>[2x]GPSGMILKRAYDVTPQKISTD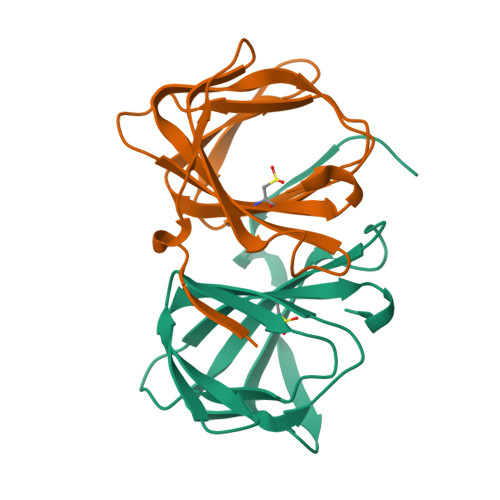KVRGVRKRVLIGLKDAPNFVMRLFTVEPGGLIDRHSHPWEHEIFVLKGKLTVLKEQGEETVEEGFYIFVEPNEIHGFRNDTDSEVEFLCLIPKEGGE> GASAPMVKIYTKNGDKGQTRIIGKQILYKNDPRVAAYGEVDELNSWVGYTKSLINSHTQVLSNELEEIQQLLFDCGHDLATPADDERHSFKFKQEQPTVWLEEKIDNYTQV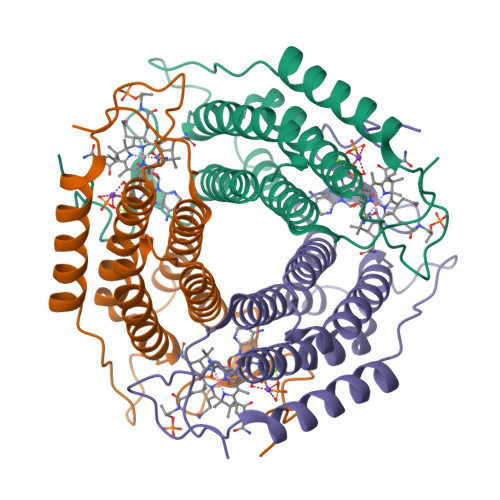VPAVKKFILPGGTQLASALHVARTITRRAERQIVQLMREEQINQDVLIFINRLSDYFFAAARYANYLEQQPDMLYRNSKDVFR2-[5-(4-carbamimidoylphenyl)thiophen-2-yl]-1H-indole-6-carboximidamide | C20 H17 N5 S | 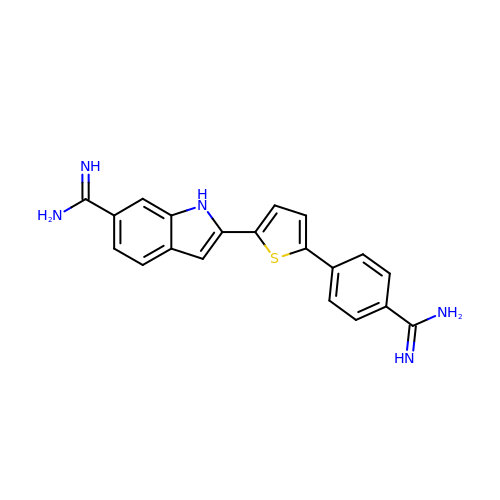SLHMDSOFLPLMCD-UHFFFAOYSA-N>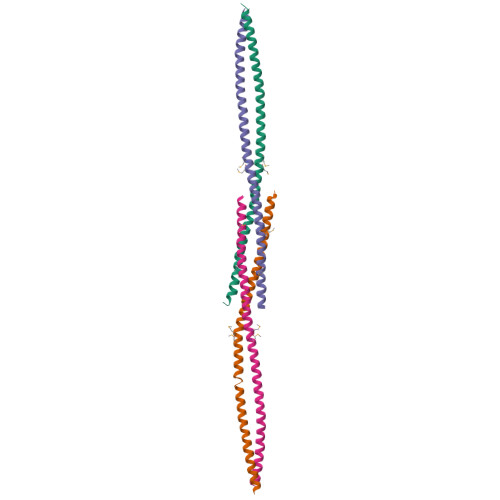[4x]GIDPFTKANSEACRDGLRAVMECRNVTHLLQQELTEAQKGFQDVEAQAATCNHTVMALMASLDAEKAQGQKKVEELEGEITTLNHKLQDASAEVERLRRENQVLSVRIADKK> MDEKSTKIIMWLKKMFGDKPLPPYEVNTRTMEILYQLAEWNEARDKDLSLVTEDLKLKSAEVKAEAKYLQDLLTEGLGPSYTNLSRMGNNYLNQIVDSCLALELKNSSLSSYIPAVNDLSSELVAIELNNQEMEAELTSLRKKLTEALVLEKSLERDLKKAEEQCNFEKAKVEIRSQNMKKLKDKSEEYKYKIHAAKDQLSSAGMEEPLTHRSLVSLSETLTELKAQSMAAKEKLNSYLDLAPNPSLVKVKIEEAKRELKATEVELTTKVNMMEFVVPEPSKRRLK;> MSGGDRFVQTLQKLNYPKGAQLDGEDFDWLFEAVDLKPFLDWFCSAASEQNVVPDEKLQAFNTLKESGKPVLDEKALDEVLKTFSISKVPAIEEVAIEKLEEEVKALQKQKNLHIRRRNKLQMVESGNRQMCLKSKDKEEETGRAFQEVLHLLRVTNKKLNHELQSIVNGVQTLMSFFSTPETACELSSQPIFLSQLLLDKYLSLEEQSTAALTSFTKEHFFEGMSKFVEGSDENFQLVQLNVNSFGEDGTTEDKCKEMMRLQLAYICAKHKLIQMKAKSASLKVGLQWAENNASVVQDKASQKEENLKVRITSLKNETLQIENHTNSISNEKLPGLVRDNAQLLNMPIVKGDYDLQMAHQTSCSSRQDLVCDHLMKQKASFELLQLGYELELRKHRDVYRELGSIVQELKESGDKLEERLTMLSDVNLLSASKPRSNIDSKDLTSHRLYQLLDGDNTQKLFRTYDGLESVAQKLSQDIASMRDQLEVSEQEHSLLLSKLDSHLKELRDFMYPEGNTLMLTTPELSGEFHQLGSQLEKLNHITVEILGDLQLKRKMLESNKLQQIEKQLYVYFFQNEEQLKSIVGKLEAQTGGGSSA;> MAQTLQYVSSRLSMLQIDEEDLERNAQFGKVLIELCPLLGPNGGSANLNRELEETRRELLLQRKMWMRSEVIYQLVQEMLLDLQVRKLEGSLTEEERKFQDGLQQCMLVSECSRLLTADSVPPSDSTSILGLDKQDLLDLLPPNMLVLWVRDRLQKQLEEALKKKCFTFLSFHQPETDEEGDVLRAAKVLRLASTLEDEKRRLQNEQEKHQEMRALLEKQQEIYPHVLLRCLSLLRQAASELRLRAQSDIDRINAEYLEAKSNALFLKLRMEELQVLTDCYTPEKVLVHRQIRDTLEAGVKKEKQELSTSRQILSSYEFLGPEFEGLVQEYTRLKDKIKDNRWMLQELSKSLP;> MERRSLAQELKKWAVEEMGLPAQKAPSEEMLQRLFIGQCGDIWKFIIRHIHSHRTVRKIEGNLLWYQQLQHTEAQRTAEEEQQQRRKQLCKEILELRAELHHLQEQIQTAEREIVGQDLNCERAQDLCRRSLLLRAFNKKREEECEALCQSNKKIQYRCEQLQEIRRASQREVMFSAVDPDLSSSTFLEPEVLRDVREVCKLRFKFLRSLHDDSISSSVHPGKEDLRSLSHQQWMSMAEKVWNTHTPNHILAALERLTLNSTQELKKLQFSQAADLSKGPSCQLKEFSEPITQSRSCNESTHLDPQETLPSFHSLIQEGWANSVKVSSELRRVQSQAQALSEHLAERIQEIHKKLSDGSEVSVLTRAAFDAELRCVILRGCRDALMQECRMLQEEAAGKKQEMKLLQQQQQNIQEACLLLDKKQKHIQILIKGNSSSKSQIRRSSVEAQKYVQDKLLPWPQEIIQESQRLQDSIQKEVKHFSAICLPALLKVSTDGFNLLPSRELSINRMSNTHAPYYGIFKGIYESVRLPLYKAPESVLSHVADMKKQLFFLRSQLSSRSEAISKTQRALQKNTNPDTDALLKSLSDHYSLELDEMVPKMQRLIQQCEKHQEYGKEVQATVMDWWEQPVQLCLPSEERGGLTLRQWRERWTVAVTALQRATGSRS;> MMAANPWSPVQPSAASLLLEKCLAAGVLSQNALDQAQLEAPCFSHAEELQRITEIKAEINQKSLELELLRLEKETADITHPLYLGQKHQALQAMNSHLEAVLREKRSLRQRLAQPVCQENLPIEASYHRFTAELLPLAVNFIEKLEIYIKTIQTIPKIPDCASNMDNALMRMESLEAEMEEVTEQILTWREQQKTAFQMNSDANSSCITAQTSYLSIENLHP;> MQSGSRPHLAWQREHMWLALQGLGFESGAEAANAGKTLVHVTFGVNMFDKPNKDAFYVVFHFLFGKLDNVRCKEVFRYCWPPLDKKRDAEFRKACCEWLKKISDEVGAGFPQVVASIFLSPGGPKFVHLLYHFARYVMLQHIKRDADAGNVFISEALQSKIQDPQKALARNKLARQKYLKVLQKENLVIEEYQRKAQLLIKQIRDMRSEHVALQNQQKLAEKVDRKISDKDENIQKTRCMWNTIMQMLKEMEKEVDVVDAVVRGNIDQYCLDGTNATLNIPNLLISRIESEMHRLQMDNVYEAGKVNLITVVQLLNEALKLVSGERSLYDCKGVRLDLQYLHGKAKFESEVLTRLRNMRHKIKREDLVSIEKIIADREREWERKWEKILGKCPFSLLKGLNPALELNPPMAPFSFDPASEEVLKSSVFCHYPASLQEYSHKEKPLKDFNQDHSGELVQRLIGATVLTRSGRKSTSSLGMATPNRRRMSLNEREFQTPTMNDRIGFQRTPSSAVQKRRADVSWKTAANSPLPCTPTPYKQDPKNMARQQLAQQVADYIVSESPRSSGGRGMELDDLLGVLSSDPFLSRKEIPRTPENLISDIRSSWRKAIQSEESLVVASPVAAPCMDSTAELESAHCSQIDLSMACFLSTSHASDQNDCSGTRIPHNTGGNKASSLHSDVVHHESIDMKSEIDSSQPEDLSLPIKENEPADKLINLLDDKKESENADTLTNPVEFIFSNQPISKLMDKTMFISVSGQENLSAHTTLSWNSSNMITSDSSSDTHEIIQFGILHETLPENAGNVSLNSTLSLGGNEEPFEKSELSDHDFTFDRKEHSSRSMEGKMDINSIRSRYEALKRTLTSLTDEEYHGDPDTSNMRFTKHKSESSLILGSDVYSPVEKVLSLDLEYLTTPSPKDRKLSLPQLISFSPETIRSEKQEDLLDVFESQDFVNPNKTFDFTSSGLDLQKSTDEGPEQLIKL;> MTGGKELGAAVELYERLQMLSCPCLEGVYLTDPQSIYELLCTPSSHRLDILQWLCSRIYPPVQEQLSSLKESQTDTKVKEIAKLCFDLMLCHFDDLDLIRGHASPFKQISFIGQLLDVIQYPDTISSNVILESLSHSTEKNVVTCIRENEELLKELFSSPHFQATLSPECNPWPADFKPLLNAEESLQKRATQSSKGKDMSNSVEALLEISSSLKALKEECVDLCSSVTDGDKVIQSLRLALTDFHQLTIAFNQIYANEFQEHCGHPAPHMSPMGPFFQFVHQSLSTCFKELESIAQFTETSENIVDVVRERHQSKEKWAGSTISTLCEKMKELRQSYEAFQQSSLQD;> MSEAGVAPIEDGSQNSSGGSSGDAALKKSKGGAKVVKSRYMQIGRSKVSKNSLANTTVCSGGKVPERGSGGTPTRRSLAPHKAKITAAVPLPALDGSIFTKEDLQSTLLD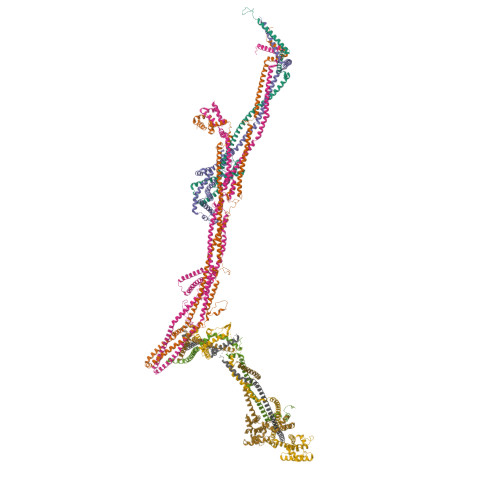GHRIARPDLDLSVINDRTLQKITPRPVVTSEQKKPKRDTTPVNLVPEDMVEMIESQTLLLTYLTIKMQKNLFRLEEKAERNLLLVNDQKDQLQETIHMMKRDLTLLQREERLRDLIEKQDEVLTPVVTSKDPFKDNYTTFATALDSTRHQLAIKNIHITGNRHRYLEELQKHLAITKSLLEEIMPSHASENAESFDTIKDLENIVLKTDEELARSFRQILDLSFKVNKEISLQSQKAVEETCESALVRQWYFDGSLP1-IODOHEXADECANE | 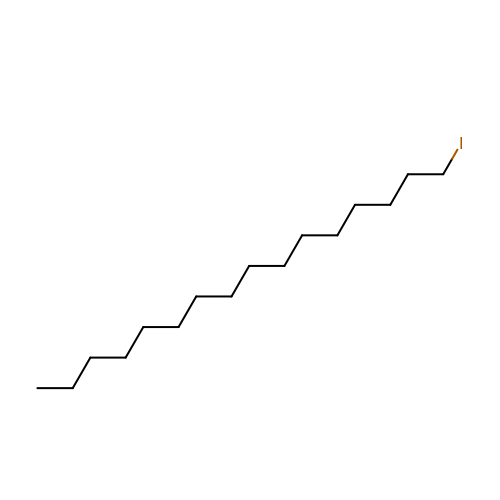C16 H33 I | KMWHQYDMBYABKL-UHFFFAOYSA-N>[12x]MKTINSVDTKEFLNHQVANLNVFTV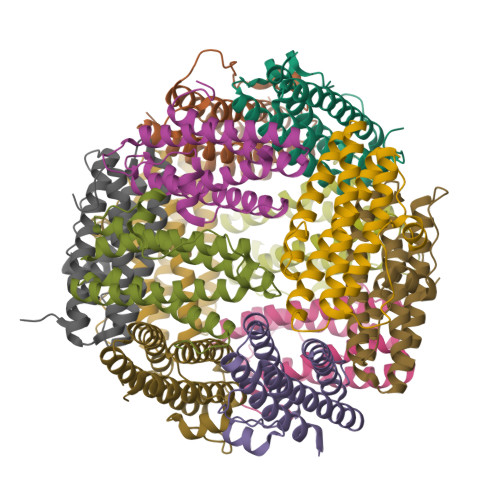KIHQIGWYMRGHNFFTLGEKMDDLYSEFGEQMDEVAERLLAIGGSPFSTLKEFLENASVEEAPYTKPKTMDQLMEDLVGTLELLRDEYKQGIELTDKEGDDVTNDMLIAFKASIDKHIWMFKAFLGKAPLE>[6x]SNAMIKQLFTHTQTVTSEFIDHNNHMHDANYNIIFSDVVNRFNYSHGLSLKERENLAYTL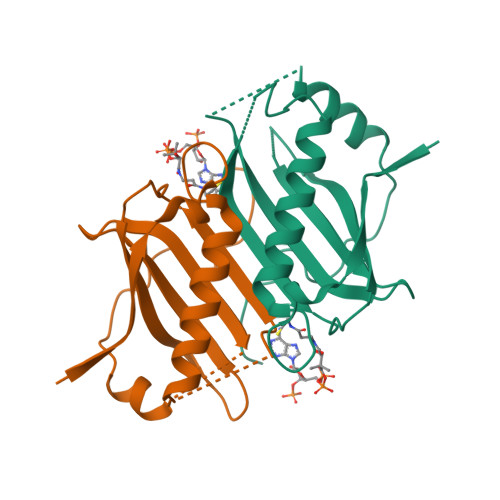FTLEEHTTYLSELSLGDVFTVTLYIYDYDYKRLHLFLTLTKEDGTLASTNEVMMMGINQHTRRSDAFPESFSTQIAHYYKNQPTITWPEQLGHKIAIPHKGALK> MASAAVANYEEEIVRPVADFSPSLWGDQFLSFSIDNQVAEKYAKEIEALKEQTRNMLLATGMKLADTLNLIDTIERLGISYHFEKEIDDILDQIYNQNSNCNDLCTSALQFRLLRQHGFNISPEIFSKFQDENGKFKESLASDVLGLLNLYEASHVRTHADDILEDALAFSTIHLESAAPHLKSPLREQVTHALEQCLHKGVPRVETRFFISSIYDKEQSKNNVLLRFAKLDFNLLQMLHKQELAQVSRWWKDLDFVTTLPYARDRVVECYFWALGVYFEPQYSQARVMLVKTISMISIVDDTFDAYGTVKELEAYTDAIQRWDINEIDRLPDYMKISYKAILDLYKDYEKELSSAGRSHIVCHAIERMKEVVRNYNVESTWFIEGYTPPVSEYLS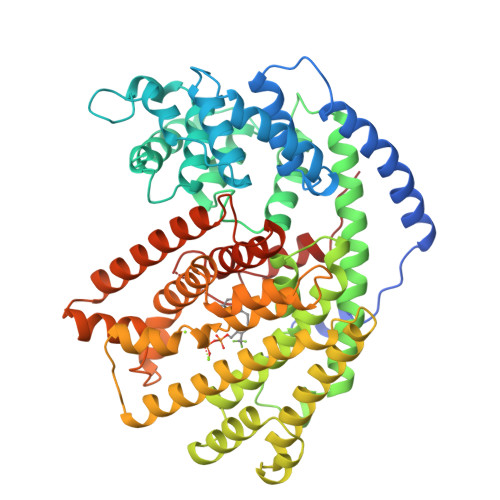NALATTTYYYLATTSYLGMKSATEQDFEWLSKNPKILEASVIICRVIDDTATYEVEKSRGQIATGIECCMRDYGISTKEAMAKFQNMAETAWKDINEGLLRPTPVSTEFLTPILNLARIVEVTYIHNLDGYTHPEKVLKPHIINLLVDSIKI4-HYDROXYBENZYL COENZYME A | C28 H42 N7 O17 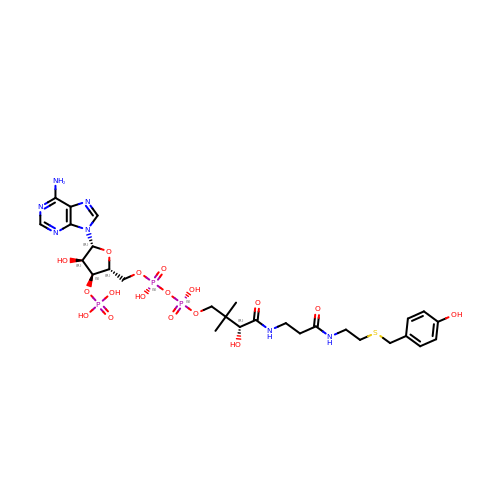P3 S | FZQUTWRNQJPTSH-SXQYHYLKSA-N> MSVIKMTDLDLAGKRVFIRADLNVPVKDGKVTSDARIRASLPTIELALKQGAKVMVTSHLGRPTEGEYNEEFSLLPVVNYLKDKLSNPVRLVKDYLDGVDVAEGELVVLENVRFNKGEKKDDETLSKKYAALCDVFVMDAFGTAHRAQASTHGIGKFADVACAGPLLAAELDALGKALKEPARPMVAIVGGSKVSTKLTVLDSLSKIADQLIVGGGIANTFIAA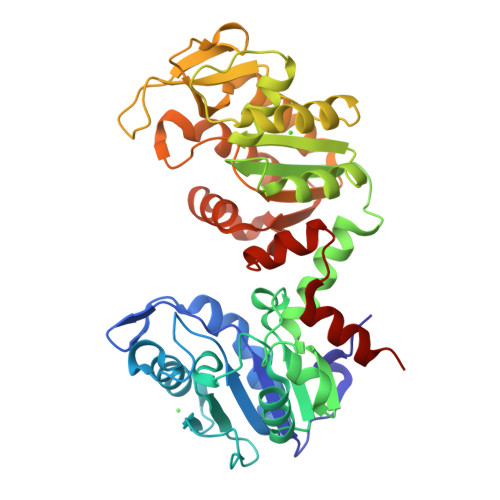QGHDVGKSLYEADLVDEAKRLLTTCNIPVPSDVRVATEFSETAPATLKSVNDVKADEQILDIGDASAQELAEILKNAKTILWNGPVGVFEFPNFRKGTEIVANAIADSEAFSIAGGGDTLAAIDLFGIADKISYISTGGGAFLEFVEGKVLPAVAMLEERAKK>[4x]AEAGITGTWYNQLGSTFIVTAGA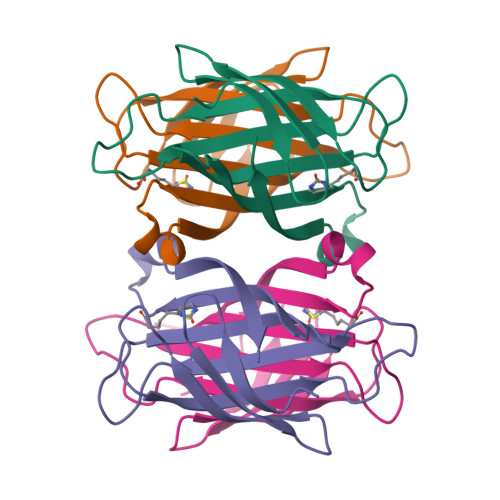DGALTGTYESAVGNAESRYVLTGRYDSAPATDGSGTALGWTVAFKNNYRNAHSATTWSGQYVGGAEARINTQWLLTSGTTEANAWKSTLVGHDTFTKVKPSAAS(((2S,3R,4S,5R,6R)-3,4,5-trihydroxy-6-(hydroxymethyl)tetrahydro-2H-pyran-2-yl)methyl)phosphonic 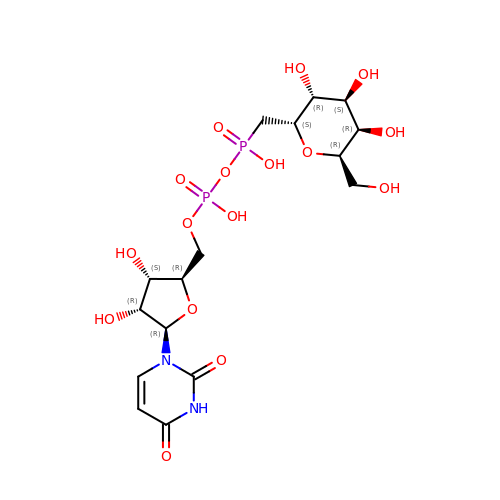(((2R,3S,4R,5R)-5-(2,4-dioxo-3,4-dihydropyrimidin-1(2H)-yl)-3,4-dihydroxytetrahydrofuran-2-yl)methyl phosphoric) anhydride | C16 H26 N2 O16 P2 | WUPLBUVQIJIOHV-PPSAJGQHSA-N9-deazaguanosine-5'-monophosphate 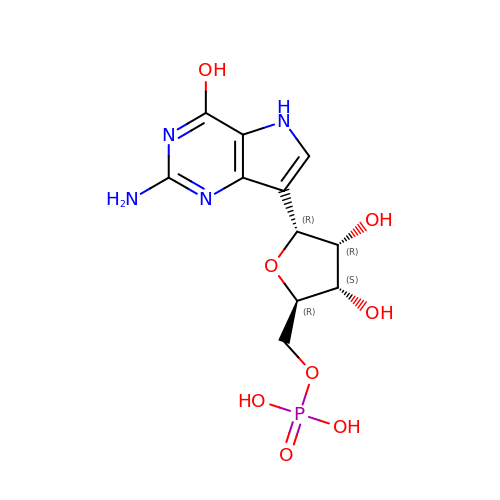| C11 H15 N4 O8 P | OHDNVDXQRZLJEP-XCBZGROMSA-N> MHHHHHHHHHHSGQNLYFQGHMATFISVQLKKTSEVDLAKPLVKFIQQTYPSGGEEQAQYCRAAEELSKLRRAAVGRPLDKHEGALETLLRYYDQICSIEPKFPFSENQICLTFTWKDAFDKGSLFGGSVKLALASLGYEKSCVLFNCAALASQIAAEQ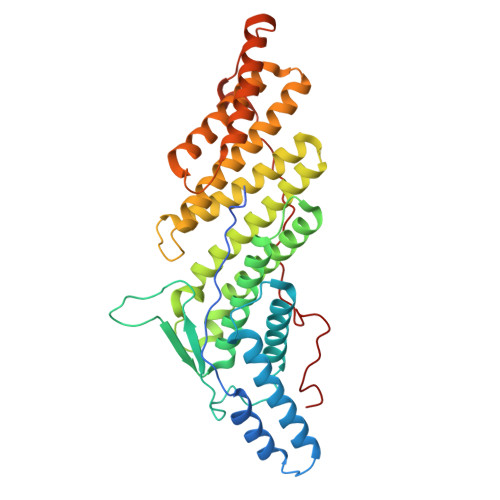NLDNDEGLKIAAKHYQFASGAFLHIKETVLSALSREPTVDISPDTVGTLSLIMLAQAQEVFFLKATRDKMKDAIIAKLANQAADYFGDAFKQCQYKDTLPKEVFPVLAAKHCIMQANAEYHQSILAKQQKKFGEEIARLQHAAELIKTVASRYDEYVNVKDFSDKINRALAAAKKDNDFIYHDRVPDLKDLDPIGKATLVKSTPVNVPISQKFTDLFEKM> MAFELFTPLFNKIDQTTATYVTDISSRAIAAITPVVSVGLTLGFITYGWLIIRGAVEMPVAEFLNRCLRIGIIVSIALAGGLYQGEIANAITTVPDELASALLGNPTQGASAAALVDQSAQQGFDRASEAFEEAGFFSSDGLLYGLFGIIIL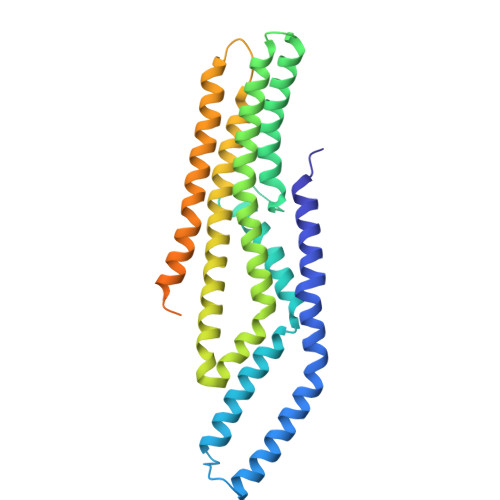LATGLLAAIGGAFLLLAKIALALLAGLGPLFILALIWQPTHRFFDQWAQQVLNYGLLIVLFAAVFGLLMQIFGSYMADLRFDGAQNVAYAIGGSVILSIVSIVLLMQLPSIASGLAGGIGLGYMWELRSMRSGAGAAMRGGRAMARGARAAPGAARGAAVGAANMAKTVATGGAGVARAAAGYFRGRKAG>[3x]CAAAGAAA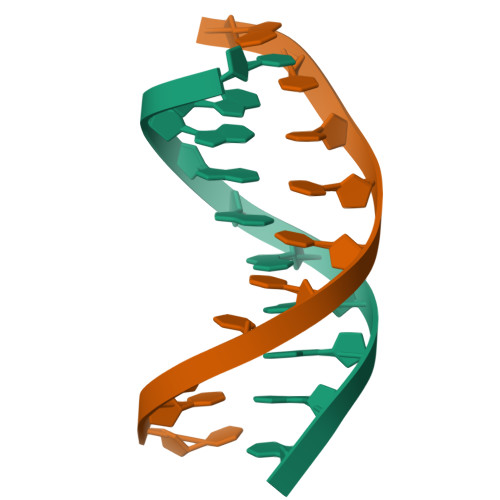AG;>[3x]CTTTTCTTTG> MAHHHHHHMVVLLYSQASWDQRSKADALVLPFWMKNSKAQEAAVVDEDYKLVYQNALSNFSGKKGETAFLFGNDHTKEQKIVLLGLGKSEEVSGTTVLEAYAQATTVLRKAKCKTVNILFPTISQLRFSVEEFLTNLAAGVLSLNYNYPTYHKVDTSLPFLEKVTVIGIVSKVGDKIFRKEESLFEGVYLTRDLVNTNADEVTPEKLAAVAKGLAGEFASLDVKILDRKAILKEKMGLLAAVAKGAAVEPRFIVLDYQGKPKSKDRTVLIGKGVTFDSGGLDLKPGKAMITMKEDMAGAATVLGIFSALASLELPINVTGIIPATENAIGSAAYKMGDVYVGMTGLSV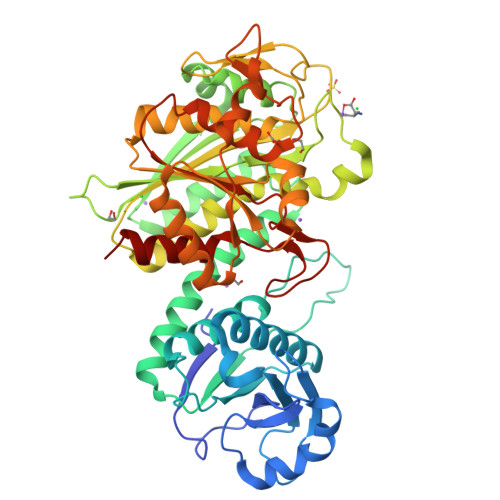EIGSTDAEGRLILADAISYALKYCNPTRIIDFATLTGAMVVSLGESVAGFFANNDVLARDLAEASSETGEALWRMPLVEKYDQALHSDIADMKNIGSNRAGSITAALFLQRFLEDNPVAWAHLDIAGTAYHEKEELPYPKYATGFGVRCLIHYMEKFLSK> MDNTGKLEKQLVTLNDGLPKKPAKEIIEELKHHLYQDFQKFFSEEKKQQYQNNFALFDRDNDKYINLSELKELLTSVNITFPDDELEELYNEFCLTSPEADGI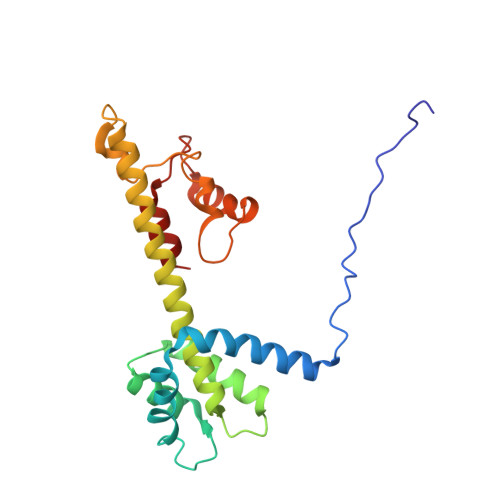NEDAVFIIVSKKIRDNDKDEQLTQAFKLVEKAVNDELAKTPNETKEQEGYIRVEQFKELLMTLGNRWSEEQANEFLKDINPKSDERINYLDVVKKLMKR1-(O-carboxy-phenylamino)-1-deoxy-D-ribulose-5-phosphate 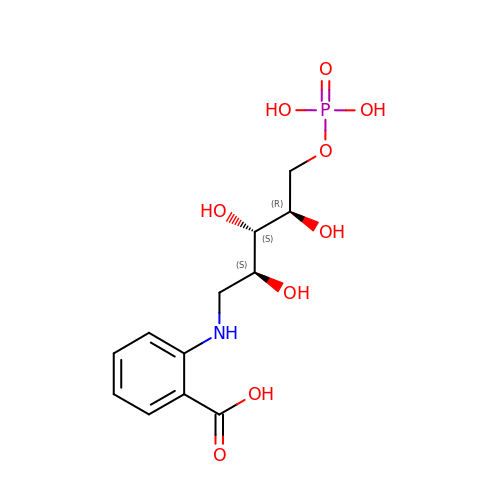| C12 H18 N O9 P | AULMJMUNCOBRHC-AXFHLTTASA-N> MHHHHHHMPLEPHFMPDFLGHAENPLREEEWARLNETVIQVARRSLVGRRILDIYGPL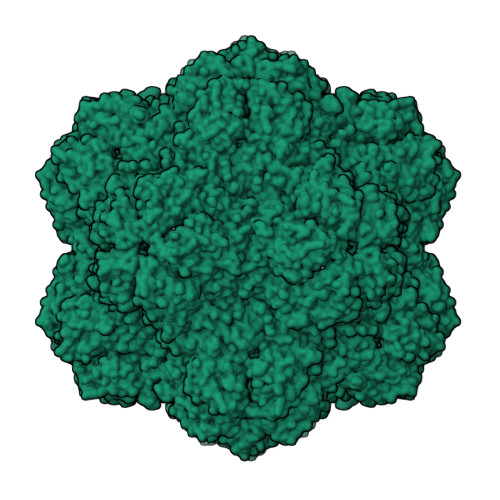GAGVQTVPYDEFQGVSPGAVDIVGEQETAMVFTDARKFKTIPIIYKDFLLHWRDIEAARTHNMPLDVSAAAGAAALCAQQEDELIFYGDARLGYEGLMTANGRLTVPLGDWTSPGGGFQAIVEATRKLNEQGHFGPYAVVLSPRLYSQLHRIYEKTGVLEIETIRQLASDGVYQSNRLRGESGVVVSTGRENMDLAVSMDMVAAYLGASRMNHPFRVLEALLLRIKHPDAICTLEGAGATERR> MGSSHHHHHHSSGRENLYFQGMATITLERDGLQLVGTREEPFGEIYDMAIIFHGFTANRNTSLLREIANSLRDENIASVRFDFNGHGDSDGKFENMTVLNEIEDANAILNYVKTDPHVRNIYLVGHAQGGVVASMLAGLY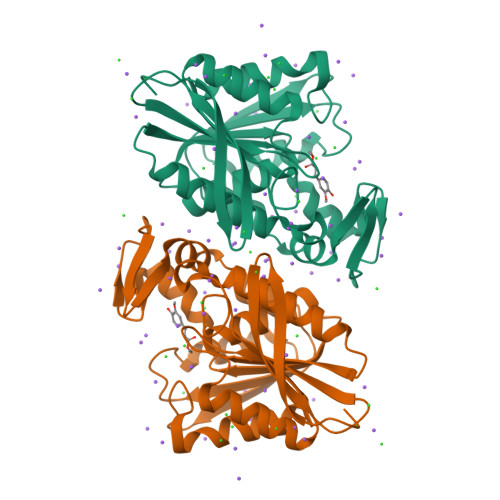PDLIKKVVLLAPAATLKGDALEGNTQGVTYNPDHIPDRLPFKDLTLGGFYLRIAQQLPIYEVSAQFTKPVCLIHGTDDTVVSPNASKKYDQIYQNSTLHLIEGADHCFSDSYQKNAVNLTTDFLQ>GASSSSESLSIIDVASDQNLFQTFIKEWRCKKRFSISLACEKIRSLTSSKTGFPIKGCDDTLVVGLAVCWGGRDAYYFSLQKESLDPSLTLKDRMWYLQSCLRKESDKECSVVIYDFIQSYKILLLSCGISLEQSYEDPKVACWLLDPDSQEPTLHSIVTSFLPHELPLLEGMETSQGIQSLGLNAGSEHSGRYRASVESILIFNSMNQLNSLLQKENLQDVFRKVEMPSQYCLALLELNGIGFSTAECESQKHIMQAKLDAIETQAYQLAGHSFSFTSSDDIAEVLFLELKLPPNRELGRQFSTSKDVLNKLKALHPLPGLILEWRRITNAITKVVFPLQREKCLNPFLGMERIYPVSQSHTATGRITFTEPNIQNVPRDFEIKMPTLADRGMPF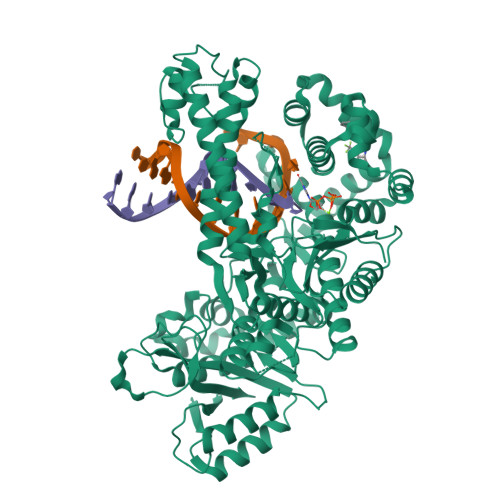SISMRHAFVPFPGGSILAADYSQLELRILAHLSHDRRLIQVLNTGADVFRSIAAEWKMIEPESVGDDLRQQAKQICYGIIYGMGAKSLGEQMGIKENDAACYIDSFKSRYTGINQFMTETVKNCKRDGFVQTILGRRRYLPGIKDNNPYRKAHAERQAINTIVQGSAADIVKIATVNIQKQLETFHSTFKSHGHREGMLQSDQTGGMFCPIRGGFFILQLHDELLYEVAEEDVVQVAQIVKNEMESAVKLSVKLKVKVKIGASWGELKDFDV[2x]>AQYEDGKQYTTLEKPVAGAPQVLAFFSFFCPHCYQFEEVLHISDNVK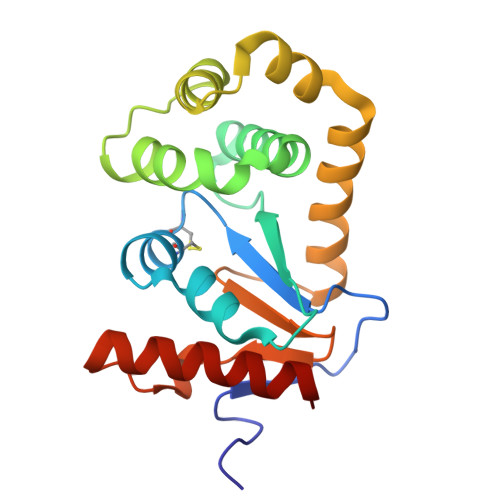KKLPEGVKMTKYHVNFMGGDLGKDLTQAWAVAMALGVEDKVTVPLFEGVQKTQTIRSASDIRDVFINAGIKGEEYDAAWNSFVVKSLVAQQEKAAADVQLRGVPAMFVNGKYQLNPQGMDTSNMDVFVQQYADTVKYLSEKK[4x]> APGQKECDNALRQLETVRELLENPVQPINDMSYFGCLDSVMENSKVLGEAMTGISQNAKNGNLPEFGDAIATASKALCGFTEAAAQAAYLVGVSDPNSQAGQQGLV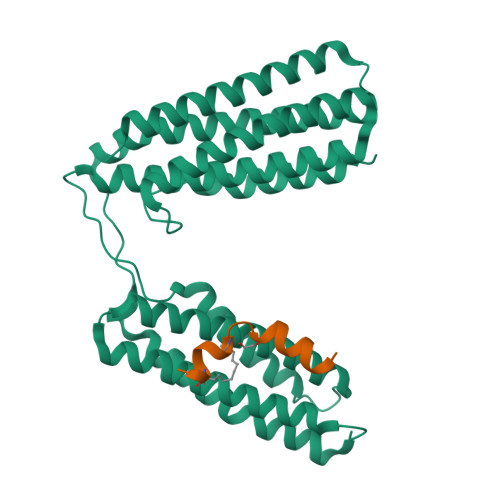EPTQFARANQAIQMACQSLGEPGCTQAQVLSAATIVAKHTSALCNSCRLASARTANPTAKRQFVQSAKEVANSTANLVKTIKALDGDFTEENRAQCRAATAPLLEAVDNLSAFASNPEFSSVPAQISPEGRAAMEPIVISAKTMLESAGGLIQTARALAVNPRDPPRWSVLAGHSRTVSDSIKKLITSMRDKAPG;> DIDQMFSTLLGELDLLLQS>[2x]MGGPAFEFAVAMMKRNSSTVKTEYGEFTMLGIYDRWAVLPRHAKPGPTILMNDQEVAVLAAKELADKDGTNLELTLLKLNRNEKFRDIRGFLAKEEV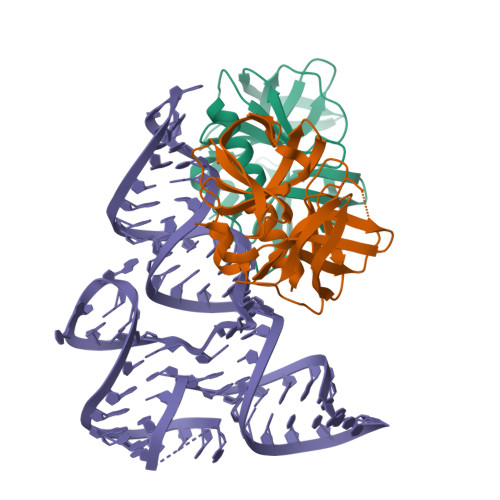EVNEAVLAINTSKFPNMYIPVGQVTEYGFLNLGGTPTKRMLMYNFPTRAGQAGGVLMSTGKVLGIHVGGNGHQGFSAALLKHYFNDEQLEHHHHHH> MPKALRFLGWPVLVGVLLALLIIQHNPELV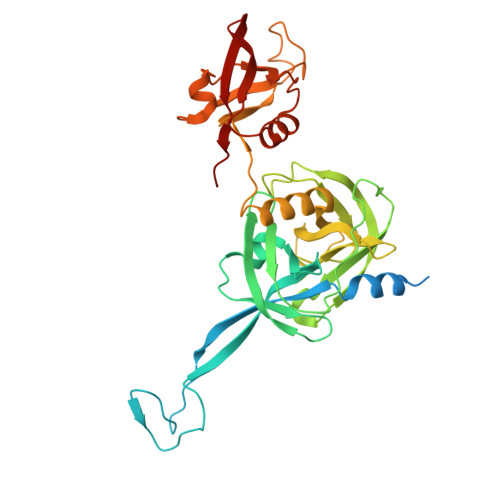GLPRQEVHVEQAPLLSRLQEGPVSYANAVSRAAPAVANLYTTKMVSKPSHPLFDDPMFRRFFGDNLPQQKRMESSLGSAVIMSAEGYLLTNNHVTAGADQIIVALRDGRETIAQLVGSDPETDLAVLKIDLKNLPAMTLGRSDGIRTGDVCLAIGNPFGVGQTVTMGIISATGRNQLGLNTYEDFIQTDAAINPGNSGGALVDAAGNLIGINTAIFSKSGGSQGIGFAIPTKLALEVMQSIIEHGQVIRGWLGVEVKALTPELAESLGLGETAGIVVAGVYRDGPAARGGLLPGDVILTIDKQEASDGRRSMNQVARTRPGQKISIVVLRNGQKVNLTAEVGLRPPP>MSQLEHNIGLSIFEPVAKHRANRIVCTIGPSTQSVEALKNLMKSGMSVARMNFSHGSHEYHQTTINNVRAAAAELGLHIGIALDTKGPEIRTGLFKDGEVSFAPGDIVCVTTDPAYEKVGTKEKFYIDYPQLTNAVRPGGSIYVDDGVMTLRVVSKEDDRTLKCHVNNHHRLTDRRGINLPGCEVDLPAVSEKDRKDLEFGVAQGVDMIFASFIRTAEQVREVRAALGEKGKDILIISKIENHQGVQNIDSIIEASNGIMVARGDLGVEIPAEKVCVAQMCIISKCNVVGKPVICATQMLESMTSNPRPTRAEVSDVANAVLNGADCVMLSGETAKGKYPNEVVQYMARICVEAQSATHDTVMFNSIKNLQKIPMCPEEAVCSSAVASAFEVQA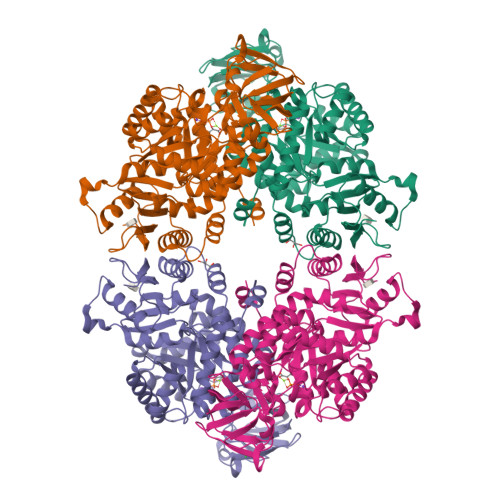KAMLVLSNTGRSARLISKYRPNCPIICVTTRLQTCRQLNVTRSVVSVFYDAAKSGEDKDKEKRVKLGLDFAKKEKYASTGDVVVVVHADHSVKGYPNQTRLIYLP[2x]>MHHHHHHTEIVADKTVEVVKNAIETADGALDLYNKYLDQVIPWQTFDETIKELSRFKQEYSQAASVLVGDIKTLLMDSQDKYFEATQTVYEWCGVATQLLAAYILLFDEYNEKKASAQKDILIKVLDDGITKLNEAQKSLLVSSQSFNNASGKLLALDSQLTNDFSEKSSYFQSQVDKIRKEAYAGAAAGVVAGPFGLIISYSIAAGVVEGKLIPELKNKLKSVQNFFTTLSNTVKQANKDIDAAKLKLTTEIAAIGEIKTETETTRFYVDYDDLMLSLLKEAAKKMIN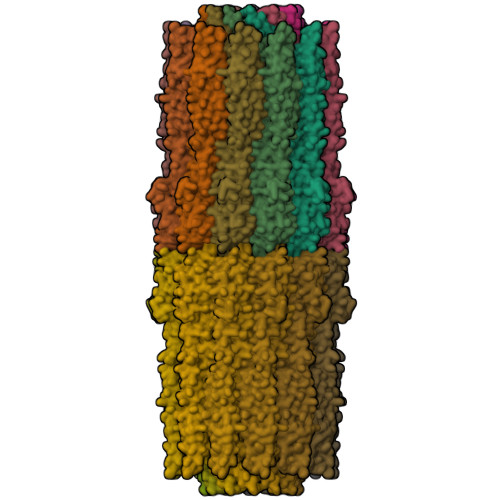TCNEYQKRHGKKTLFEVPEV[24x]>[4x]MNPAAEAEFNILLATDSYKVTHYKQYPPNTSKVYSYFECREKKTENSKLRKVKYEETVFYGLQYILNKYLKGKVVTKEKIQEAKDVYKEHFQDDVFNEKGWNYILEKYDGHLPIEIKAVPEGFVIPRGNVLFTVENTDPECYWLTNWIETILVQSWYPITVATNSREQKKILAKYLLETSGNLDGLEYKLHDFGYRGVSS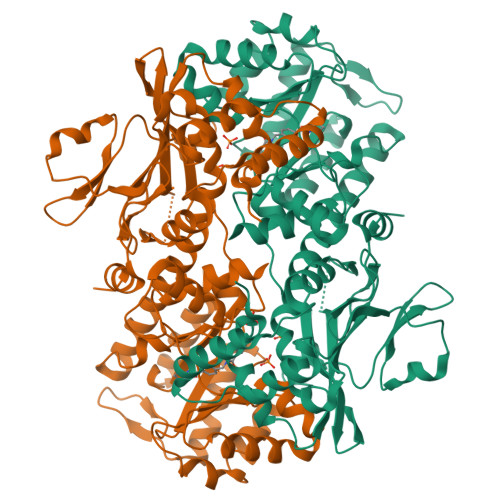QETAGIGASAHLVNFKGTDTVAGLALIKKYYGTKDPVPGYSVPAAEHSTITAWGKDHEKDAFEHIVTQFSSVPVSVVSDSYDIYNACEKIWGEDLRHLIVSRSTQAPLIIRPDSGNPLDTVLKVLEILGKKFPVTENSKGYKLLPPYLRVIQGDGVDINTLQEIVEGMKQKMWSIENIAFGSGGGLLQKLTRDLLNCSFKCSYVVTNGLGINVFKDPVADPNKRSKKGRLSLHRTPAGNFVTLEEGKGDLEEYGQDLLHTVFKNGKVTKSYSFDEIRKNAQLNIELEAAHH> MTIAPITGTIKRRVIMDIVLGF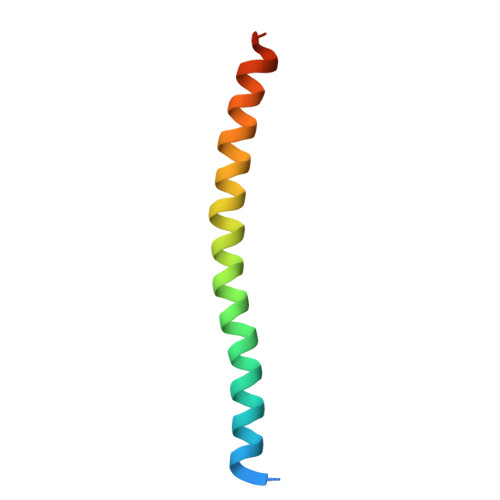SLGGVMASYWWWGFHMDKINKREKFYAELAERKKQEN>[2x]VILTGNSSLCPISGWAIYSKDNGIRIGSKGDVFVIREPFISCSHLECRTFFLTQGALLNDKHSNGTVKDRSPYRTLMSCPVGEAPSPYNSRFESVAWSASACHDGMGWLTIGISGPDNGAVAVLKYNGIITDTIKSWRNNILRTQESECACVNGSCFTIMTDGPSNGQASYKILKIEKGKVTKSIELNAPNYHYEECSCYPD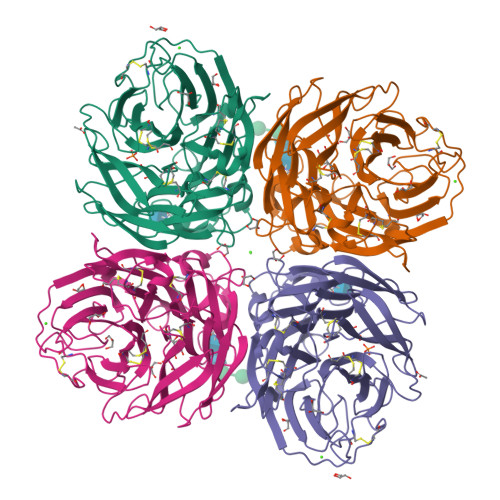TGKVMCVCRDNWHGSNRPWVSFDQNLDYQIGYICSGVFGDNPRPNDGTGSCGPVSSNGANGIKGFSFRYDNGVWIGRTKSTSSRSGFEMIWDPNGWTETDSSFSVRQDIVAITDWSGYSGSFVQHPELTGLDCMRPCFWVELIRGQPKENTIWTSGSSISFCGVNSDTVGWSWPDGAELPFSI> IVGGQECKDGECPWQALLINEENEGFCGGTILSEFYILTAAHCLYQAKRFKVRVGDRNTAAEEGGEAVHEVEVVIKHNRFTKETYDFDIAVLRLKTPITFRMNVAPACLPERDWAESTLMTQKTGIVSGFGRTHEK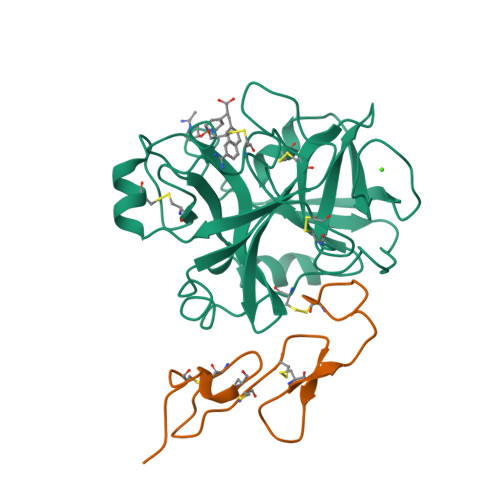GRQSTRLKMLEVPYVDRNSCKLSSSFIITQNMFCAGYDTKQEDACQGDSGGPHVTRFKDTYFVTGIVSWGEGCARKGKYGIYTKVTAFLKWIDRSMKTRGLPKAKSHAPEVITSSPLK;> YKDGDQCETSPCQNQGKCKDGLGEYTCTCLEGFEGKNCELFTRKLCSLDNGDCDQFCHEEQASVVCSCARGYTLADNGKACIPTGPYPCGKQTLER4-(2-{[(1R)-2-(1H-indol-3-yl)-2-oxo-1-phenylethyl]amino}ethyl)benzene-1-sulfonamide 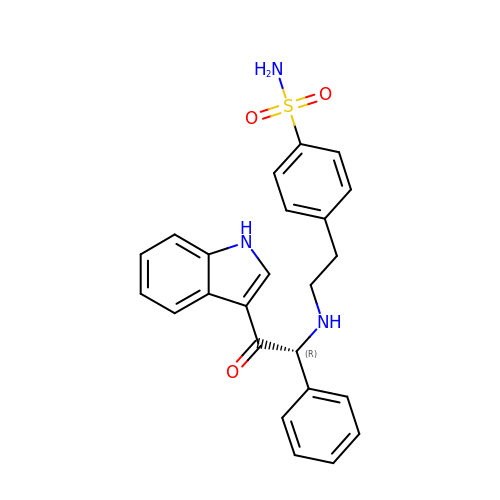| C24 H23 N3 O3 S | GLJNFDHGTNKTJR-HSZRJFAPSA-N> GPSGSIIATDNVLFTPRDKLTVEELEQFQSKKFTLGKIPLK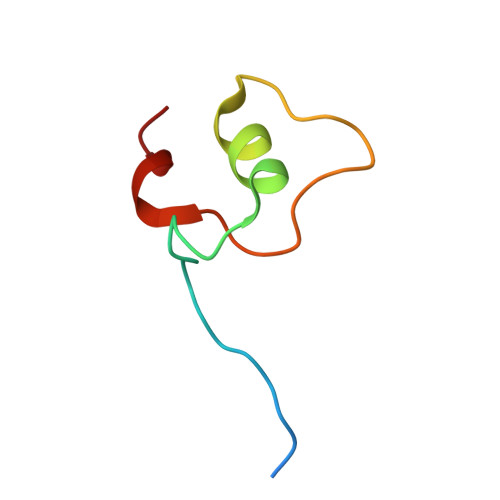PPPLELLNV> RMERDTFGEIAVPAARLWGAQTQRSLQNFKISTEKQSPELIHALALIKRAAAAVNLELGVLAQDKANAIVAAADEIIAGRHADEFPLAVWQTGSGTQTNMNLNEVIANRASELLGGERGESRAVHPNDDVNRGQSSNDVFPTAMHIAAARAIVDHLLPALRTLRATLDAKAAAFADIVKIGRTHLQDATPLTLGQEFSGYVAQLDQGIRHVEAALPHLYELAQGGTAVGTGLNAHPKFAAGVAAEIGRLTGLPFVSAPNKFEVMAAADALVFAHGALKTVAASLMKIANDIRWLASGPRCGLGELSIPENEPGSSIMPGKVNPTQSEAVTM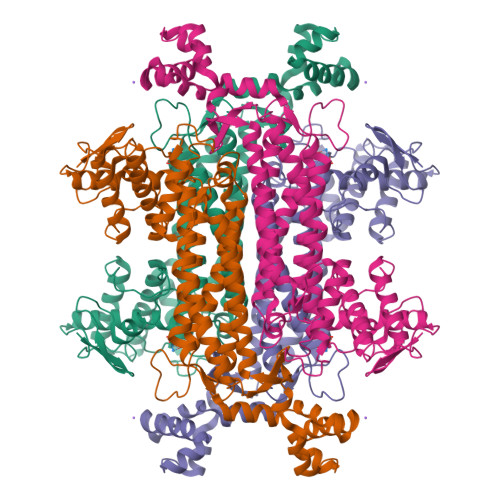LCCQVFGNDVAVNFGGASGNFELNVFRPMIAHNVLQSVRLLADGAQGFNDHCAVGIEPNRARIDALLNESLMLVTALNPHIGYDKAAQIAKKAHKEGTTLKAAALALGYVTDAQFDEWVRPEHMVGNR>HHHHHHMKFTVEREHLLKPLQQVSGPLGGRPTLPILGNLLLQVADGTLSLTGTDLEMEMVARVALVQPHEPGATTVPARKFFDICRGLPEGAEIAVQLEGERMLVRSGRSRFSLSTLPAADFPNLDDWQSEVEFTLPQATMKRLIEATQFSMAHQDVRYYLNGMLFETEGEELRTVATDGHRLAVCSMPIGQSLPSHSVIVPRKGVIELMRMLDGGDNPLRVQIGSNN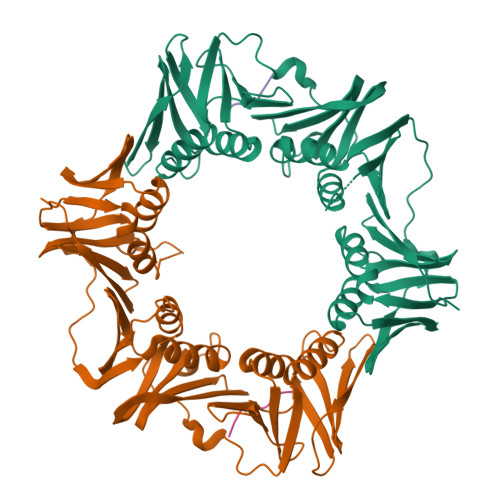IRAHVGDFIFTSKLVDGRFPDYRRVLPKNPDKHLEAGCDLLKQAFARAAILSNEKFRGVRLYVSENQLKITANNPEQEEAEEILDVTYSGAEMEIGFNVSYVLDVLNALKCENVRMMLTDSVSSVQIEDAASQSAAYVVMPMRL[2x];>[2x]CQGVAQLNLFDD> PLPPLP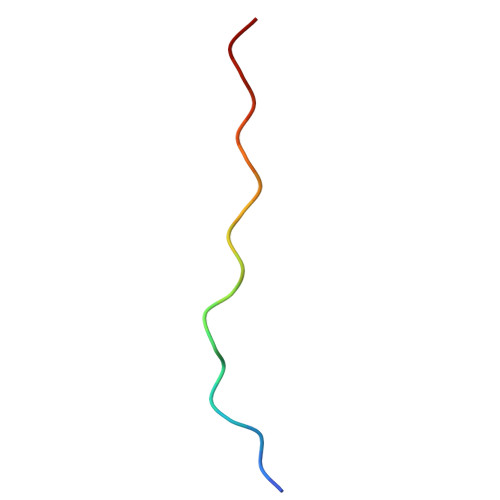PLPPLPPLPPLPP2-(5-bromo-1H-indol-3-yl)-N-hydroxyacetamide | C10 H9 Br N2 O2 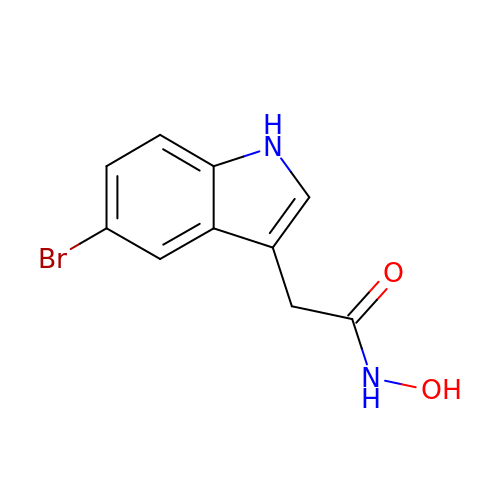| ZDQORGWUODGWFT-UHFFFAOYSA-N The fold of CrataBL consists of a β-trefoil, typical for this protein family. To conclude, the sequence and three-dimensional structure of CrataBL show extensive similarity to protease inhibitors of the Kunitz-type, although the inhibitory activity is weak (in the micromolar range). A number of its biological properties have been characterized, including delay in clot formation by impairing the intrinsic pathway of coagulation cascade. In addition, CrataBL was shown to exhibit anti-inflammatory, analgesic, insecticidal, and anti-tumor activities.

The three-dimensional structure of CrataBL was determined in two crystal forms. Both of them were in space group C2 and contained two molecules in the asymmetric unit, but the unit cell parameters and crystal packing were different. Further analysis of glycosylation by mass spectrometry and protein sequence determination has shown the presence of N-linked oligosaccharides at Asn27 and Asn57. However, it is not clear whether the dimer observed in both crystal forms of CrataBL is biologically significant. There is no particular need for dimerization of a protease inhibitor, since Kunitz-P type inhibitors form 1∶1 complexes with their target enzymes. Since we were not able to obtain crystals of CrataBL with a target protease such as trypsin, the location of the reactive loop may only be predicted. However, the observation that CrataBL is slowly cleaved by trypsin between serines 58 and 59, located on a loop that is involved in direct interaction with the active site residues in trypsin and other serine proteases, lends credence to this assumption. Thus the detailed structural basis of the inhibition mode by CrataBL still needs to be verified.

>[2x]AILTGVPYYILPSTSRAGFSPDNLRKNTSQPSCPLDLITQLRFPPRIGVPVIFTPQNSSLKVVPLSHNLNIHTCSDLWFCPESKIWTVKSSSIHRGLVVTTGGTFRSLGSWFRIERHGDSYKLVHCPRGSTPCRDVGIETVGGGGRRYLAPRDRPLAVRFTRASG>HHHHHHLPNITILATGGTIAGGGDSATKSSYTVGKVGVENLVNAVPQLKDIANVKGEQVVNIGSQDMNDNVWLTLAKKINTDCDKTDGFVITHGTDTMEETAYFLDLTVKCDKPVVMVGAMRPSTSMSADGPFNLYNAVVTAADKASANRGVLVVMNDTVLDGRDVTKTNTTDVATFKSVNYGPLGYIHNGKIDYQRTPARKHTSDTPFDVSKLNELPKVGIVYNYANASDLPAKALVDAGYDGIVSAGVGNGNLYKSVFDTLATAAKTGTAVVRSSRVPTGATTQDAEVDDAKYGFVASGTLNPQKARVLLQLALTQTKDPQQIQQIFNQY[4x]

Bacterial L-asparaginases are amidohydrolases (EC 3.5.1.1) capable of deaminating L-asparagine and, with reduced efficiency, L-glutamine. Bacterial L-asparaginases are homotetrameric proteins of 140–150 kDa. Each subunit is built-up by nearly 330 amino acids and consists of two α/β domains connected by a ca 21 amino-acid-long random coil. To obtain high-quality crystals, we took advantage of the highly stable N24S L-asparaginase, which shares identical catalytic and structural properties with the wild-type enzyme, but has largely improved stability and forms highly ordered crystals.

The asymmetric unit (ASU) of apo-N24S, solved at 1.70 Å resolution, comprised 4 monomers, named A, B, C, and D. Chains A/B and C/D are associated into two independent intimate dimers. The biological unit was rebuilt using the crystallographic C2 symmetry operators. None of the protomers contained a complete electron density trace in the region corresponding to the extremely mobile active site flexible loop (ASFL). Protomer A missed residues 15–30, protomer B 16–31, protomer C 16–32, and protomer D, the most complete, 15–25. Analysis of the solvent content inside the apo-N24S-binding pocket confirms the presence of the four highly conserved water molecules (named W1–W4) that are known to coordinate and interact with the rigid part of the substrate-binding pocket. As previously observed for the wild-type apo-enzyme, in fact, the position of each of the four water molecules exactly coincides with one of the oxygen atoms of the two carboxylic groups of the bound L-ASP ligand. In ErAII, the C-domain loop establishes contacts only with G28, a residue belonging to the ASFL and not involved in the catalytic process. Such a tight contact between the two monomers in EcAII intimate dimers (present also in the enzyme apo-structure) makes the size of the opening, useful for substrate access and product exiting from the active site, quite narrow.>MDFSRFFIDRPIFAAVLSILIFITGLIAIPLLPVSEYPDVVPPSVQVRAEYPGANPKVIAETVATPLEEAINGVENMMYMKSVAGSDGVLVTTVTFRPGTDPDQAQVQVQNRVAQAEARLPEDVRRLGITTQKQSPTLTLVVHLFSPNGKYDSLYMRNYATLKVKDELARLPGVGQIQIFGSGEYAMRVWLDPNKVAARGLTASDVVTAMQEQNVQVSAGQLGAEPLPQESDFLISINAQGRLHTEEEFGNIILKTAQDGSLVRLRDVARIEMGSGSYALRSQLNNKDAVGIGIFQSPGANAIDLSNAVRAKMAELATRFPEDMQWAAPYDPTVFVRDSIRAVVQTLLEAVVLVVLVVILFLQTWRASIIPLIAVPVSVVGTFSILYLLGFSLNTLSLFGLVLAIGIVVDDAIVVVENVERNIEEGLAPLAAAHQAMREVSGPIIAIALVLCAVFVPMAFLSGVTGQFYKQFAVTIAISTVISAINSLTLSPALAALLLKPHGAKKDLPTRLIDRLFGWIFRPFNRFFLRSSNGYQGLVSKTLGRRGAVFAVYLLLLCAAGVMFKVVPGGFIPTQDKLYLIGGVKMPEGSSLARTDAVIRKMSEIGMNTEGVDYAVAFPGLNALQFTNTPNTGTVFFGLKPFDQRKHTAAEINAEINAKIAQIQQGFGFSILPPPILGLGQGSGYSLYIQDRGGLGYGALQSAVNAMSGAIMQTPGMHFPISTYQANVPQLDVQVDRDKAKAQGVSLTELFGTLQTYLGSSYVNDFNQFGRTWRVMAQADGPYRESVEDIANLRTRNNQGEMVPIGSMVNISTTYGPDPVIRYNGYPAADLIGDADPRVLSSSQAMTHLEELSKQILPNGMNIEWTDLSFQQATQGNTALIVFPVAVLLAFLVLAALYESWTLPLAVILIVPMTMLSALFGVWLTGGDNNVFVQVGLVVLMGLACKNAILIVEFARELEIQGKGIMEAALEACRLRLRPIVMTSIAFIAGTIPLILGHGAGAEVRGVTGITVFSGMLGVTLFGLFLTPVFYVTLRKLVTRRKPVQEDLPAHHHHHH[3x]

Resistance nodulation and cell division (RND) efflux pumps are secondary active antiporters that are ubiquitous across all domains of life. As part of tripartite multidrug efflux systems in Gram-negative bacteria, they span the entire cell envelope and export a broad variety of structurally and chemically unrelated toxic substrates. During drug efflux, AcrB undergoes a functional rotation where each of the three protomers sequentially cycles through the conformational states loose (L), tight (T) and open (O). Substrates can enter the PD through several channels and bind to the access pocket (AP) in the L state and the deep binding pocket (DBP) in the T state.

Given the parallels in both the phenotype and the structural characteristics of AcrB V612F and the proteins from the OqxB cluster, we decided to assess the structural characteristics of OqxB as a representative of this cluster. We were able to obtain a detergent-solubilised OqxB crystal structure in the TTO state. Thus, OqxB can also adopt an asymmetric structure next to the previously determined TTT state22 in the presence of a substrate (here: DDM). The O monomer of the TTO structure closely resembles the O state of AcrB and has an open exit channel for substrate extrusion as expected. Whereas OqxB adopts a single conformation, O*O*O*, in the absence of substrate (Apo-state), crystal structures indicated that OqxB adopts the OTT and TTT states in the presence of substrate (DDM). Further, a comparison of the porter domain of AcrB and OqxB shows that in the T states a shift of the PC2 subdomain towards the PC1 subdomain is observed in OqxB. As these subdomains flank the AP, this results in a smaller AP cleft in OqxB compared to AcrB. Additionally, the channels leading from the TMD to the DBP in OqxB have smaller bottleneck radii and are overall narrower compared to AcrB.The APOBEC3 family of single-stranded DNA (ssDNA) cytosine deaminases plays important roles in innate immunity against viruses and transposons. However, a subset of APOBEC3 proteins, most notably the nuclear-localized APOBEC3B (A3B) enzyme, is strongly implicated in causing mutations in various human cancers. Human A3B consists of tandem zinc-coordinating cytosine deaminase domains: an N-terminal domain with a pseudo active site and a C-terminal functional catalytic domain. The active site has a catalytically essential zinc ion coordinated by two cysteines (Cys284 and Cys289) and a histidine (His253), with the fourth position of tetrahedral coordination available for directly interacting with the transition state of the hydrolytic cytosine deamination reaction.

The crystals have two protein monomers in the asymmetric unit, each containing a zinc ion bound in the active site. Loops 1 and 7 of A3B(187–378)QM_Δloop3 in the new crystal form show different conformations from those observed previously. In both A and B chains of the new structures, the loop 1 residue Arg211 is flipped out and, instead, the adjacent residue Arg212 projects into the DNA-binding groove and interacts with loop 7 Tyr315. In contrast, Tyr315 in chain B shows an alternative conformation differing by a rotation about the Cα-Cβ bond, in which the Tyr315 side chain is flipped away from loop 1 (χ1 ≈ 180°, trans). Importantly, this trans conformation of Tyr315 was also observed in the open state crystal structure of the A3Bctd active site bound to a TC-containing ssDNA substrate, where the Tyr315 side chain lines a hydrophobic pocket that accommodates the –1 T base. However, in our new apo A3Bctd crystal form, Tyr315 in this alternative conformation maintains the cation-π stacking interaction with the guanidinium group of Arg212. Accordingly, Arg212 in B chain is positioned differently from that in A chain, but is still blocking the ssDNA-binding groove. Of note, the two datasets we collected using different cryo-protectants showed a slight difference in the conformation of Tyr315 in the B chain. In the new crystal form, Arg210 is released and flipped out, replaced by Arg311 that in turn occupies the pocket between α1 and Trp281. The three distinct conformations of the loops 1 and 7 observed in the apo (DNA-free) A3B(187–378)QM_Δloop3 structures collectively represent possible modes of regulated ssDNA access to the A3B active site, in which the closed state of either loop 1 or 7 (or both together) is incompatible with substrate binding.

>[2x]SEILRYLMDPDTFTSNFNNDPLVLRRRQTYLCYEVERLDNGTSVKMDQHMGFLCNESGRHAELRFLDLVPSLQLDPAQIYRVTWFISWSPCFSWGCAGEVRAFLQENTHVRLRIKAARIYDYDPLYKEALQMLRDAGAQVSIMTYDEFEYCWDTFVYRQGCPFQPWDGLEEHSQALSGRLRAILQ In such microorganisms, the majority of small molecules are taken up by members of the OprD outer membrane protein family. Here we show that OprD channels require a carboxyl group in the substrate for efficient transport, and based on this we have renamed the family Occ, for outer membrane carboxylate channels. As expected from pairwise sequence identities that range from 35%–50%, the Occ proteins share a similar architecture, with a slightly off-center constriction formed by the inward-folded extracellular loops L3 and L7 and residues in the barrel wall. The transport data demonstrate that Occ channels have a pronounced preference for substrates with a carboxyl group, due to the universal presence of a basic ladder on one side of the barrel wall.

To determine if the phylogenetic subdivision of Occ proteins exists at the structural level, we determined X-ray crystal structures for seven Occ family members (OccD2, OccD3, and OccK2–K6). The pores of the proteins within the OccK subfamily show a considerable variation in size and shape, suggesting differences in substrate preferences within subfamilies as well. The next substrate tested, pyroglutamate, has a similar activity profile compared to benzoate/glucuronate. As with benzoate/glucuronate, the channel that is most efficient in pyroglutamate uptake (OccK3) was indeed predicted to transport this and related five-membered ring compounds. OccK3-mediated transport is affected only with the cephalosporin cefotaxime. OccK3 thus appears to serve as a specific entry channel for this antibiotic, which is borne out by the liposome swelling experiments.

> GHHHHHHHENLYFQGLEDLVEDSHASLELRNFYFNRDFRQSGARDNADEWAQGFLLRLESGFSEGTVGFGVDAIGLLGFKLDSGSGSGGTGLLPADGSAGGSQDDYAKLGLTAKARVSNSLLKVGALHFKSPLVSANDTRLLPELFRGALLDVQEIDGLTLRGAHLDRNKLNSSSDYQVFSANRIGGRSDAFDFAGGDYRLTPALTASLHQGRLKDIYRQTFAGLVHTLDLGGQRSLKSDLRFARASEDGGFRELDNRAFGALFSLRLGAHAVAAGYQRISGDDPYPYIAGSDPYLVNFIQIGDFGNVDERSWQLRYDYDFGALGLPGLSFMSRYVSGDNVARGAANDGKEWERNTDLGYVVQSGPLKNLGVKWRNATVRSNFANDLDENRLILSYSLALW> MTLQKDKVIKWVRFTPPQVLAIGFFLTIIIGAVLLMLPISTTKPLSWIDALFTAASATTVTGLAVVDTGTQFTVFGQTVIMGLIQIGGLGFMTFAVLIVMILAAAIGLKERMLVQEALNQPTIGGVIGLVKVLFLFSISIELIAALILSIRLVPQYGWSSGLFASLFHAISAFNNAGFSLWPDNLMSYVGDPTVNLVITFLFITGGIGFTVLFDVMKQRRFKTFSLHTALMLTGTLMLNAIAMLTVFILEYSNPGTLGHLAAVDKLWASYFQAVTPRTAGFNSLDFGSMREGTIVFTLLLMFIGAGSASTASGIKLTTFIVILTSVIAYLRGKKETVIFRRSIKYPIIIKALAVSVTSLFIVFLGIFALTITEQAPFLQIVFETFSAFGTVGL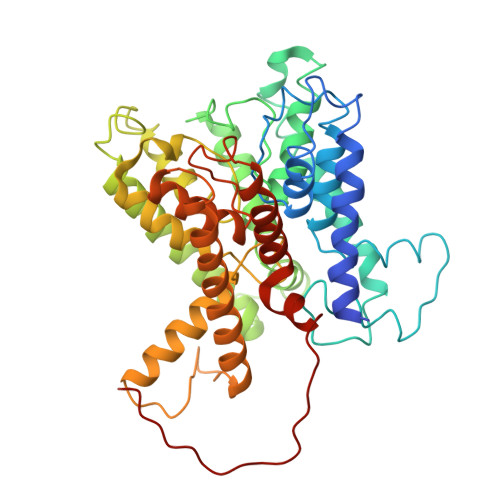TMGLTPELTTAGKCIIIVIMFIGRIGPLTFVFSFAATEQSNIRYPDGEVFTG> MSLSTIRIGGAAVNQTPIDWENNVKNILDAIEEAKNANVEILCLPELCITGYGCEDLFLTDWVAETAIEYCFEIAASCTDITVSLGLPMRIAGITYNCVCLVENGIVKGFSAKQFLANEGVHYETRWFTAWPRNHTTTFLYNDVKYPFGDVLYNVKDARIGFEICEDAWRTDRVGIRHYEKGATLVLNPSASHFAFGKSAIRYDLVIGGSERFDCTYVYANLLGNEAGRMIYDGEVLIAHKGKLIQRNDRLSFKNVNLIYADIATDSAETPETVLTQDDLEKEFEFWEATSLGLFDYMRKSRSKGFVLSLSGG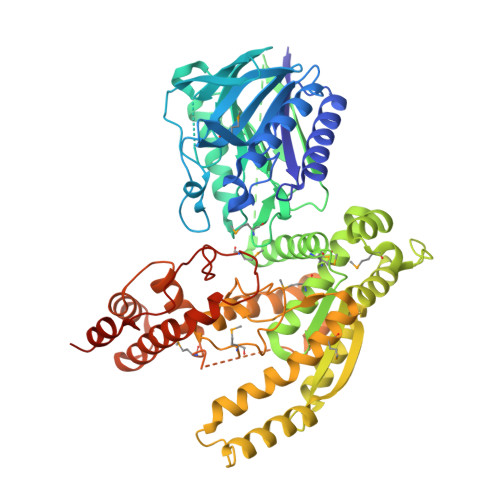ADSSACAIMVAEMIRKGLKELGLTAFLQKSNMETLFDLPALQHLPFEEQAKKITAVFLTTAYQSTRNSGDETYTSAKTLAESIGATFYNWSVDEEIEQYKATIENVIERPLTWEKDDITLQNIQARGRAPIIWMLTNVKQALLITTSNRSEGDVGYATMDGDTAGGIAPIAGVDKDFIRSWLRWAEKNRNQHGLHIVNKLAPTAELRPSEYTQTDERDLMPYDVLARIERKAIKERLSPVQVYTALLTEGPYTKNEFKYWVKKFFRLWSINQWKRERLAPSFHMDDFNIDPRSWYRFPILSSGFAKELNDLDQEGHHHHHH>GPGSELPQMVQQLNSPDQQELQSALRKLQQIAMGGNEQIQAVIDAGALPALVQLLSSP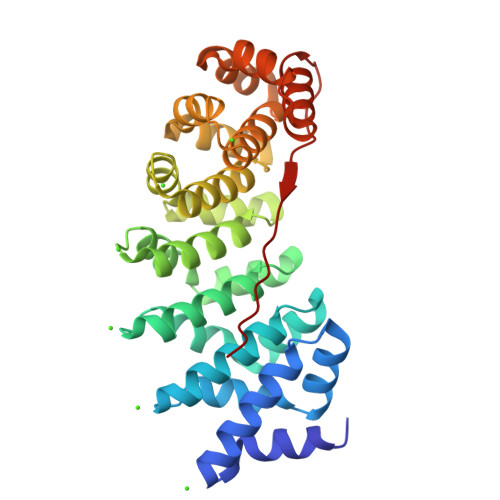NEQILASALGALANIASGGNEQIQAVIDAGALPALVQLLSSPNEQILQFALIALANIASGGNEQIQAVIDAGALPALVQLLSSPNEQILQEALWALSNIASGGNEQIQAVIDAGALPALVQLLSSPNEQILQEALWALSNIASGGNEQIQAVIDAGALPALVQLLSSPNEQILQEALWALSNIASGGNEQKQAVKEAGALEKLEQLQSHENEKIQKEAQEALEKLQSHGSGGSGKRKRKAKLSF[6x]>MRVGIKVLGCPKNEADCEVLAGVLREGGHEIVFDVKDADVVVLDTCAFIEDAKRESIDEIFSFVDAKDQYGYKLVVKGCLVQRYYEELKKEIPEVDQWIGVADPEEIANAIENGTDLVPDQPETVYRYRKRIDLEERPYAYVKISDGCDRGCTFCSIPSFKGSLRSRSIEDITREVEDLLKEGKKEIILVAQDTTSYGIDLYRKQALPDLLRRLNSLNGEFWIRVMYLHPDHLTEEIISAMLELDKVVKYFDVPVQHGSDKILKLMGRTKSSEELKKMLSSIRERFPDAVLRTSIIVGFPGETEEDFEELKQFVEEIQFDKLGAFVYSDEEGTVAFNLKEKVDPEMAKRRQEELLLLQAEISNSRLDRFVGKKLKFLVEGKEGKFLVGRTWTEAPEVDGVVFVRGKGKIGDFLEVVIKEHDEYDMW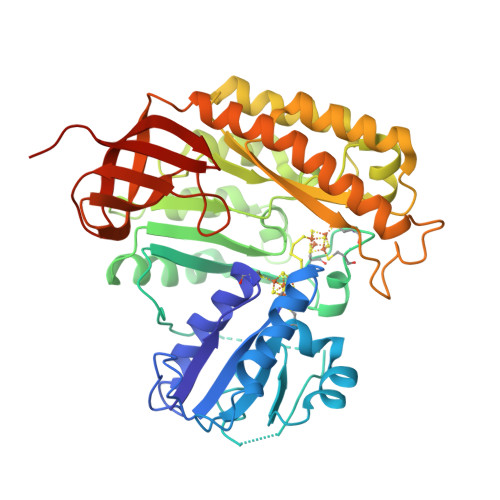GSVILEHHHHHH[2x]>GPLGSQLVVRAKFNFQQTNEDELSFS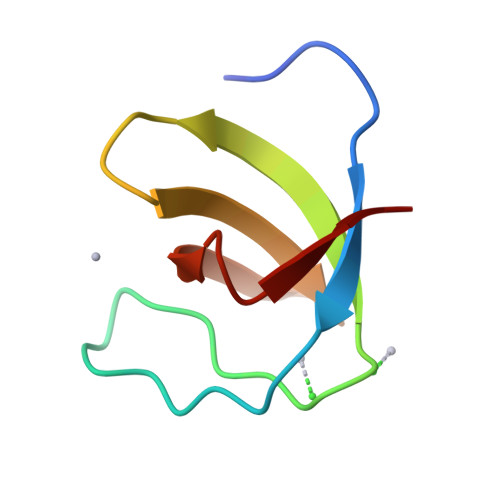KGDVIHVTRVEEGGWWEGTHNGRTGWFPSNYVREI[2x]>[2x]SNVPHKSSLPEGIRPSTVLRIRGLVPPNASRFHVNLLCGEEQGSDAALHFNPRLDTSEVVFNSKEQGSWGREERGPGVPFQRGQPFEVLIIASDDGFKAVVGDAQYHHFRHRLPLARVRLVEVGGDVQLDSVRIF

pmcHuman galectins (GAL) are oligomeric β-galactosidase-binding lectins assembled from small (∼15 kDa) protomeric carbohydrate recognition domains (CRD). Among prototype galectins, galectin-7 (GAL-7) is recognized for its preferential expression profiles in normal epithelial cells. For example, while extracellular GAL-7 can trigger apoptosis of activated T cells following binding to glycoreceptors via its GBS, it can also bind E-cadherin on epithelial cells independently of its GBS. In this work, we studied the impact of homodimer interface mutations on the induction of Jurkat T cell apoptosis, allowing us to positively and negatively modulate the biological activity of GAL-7 by designing a covalent disulfide bridge (G16C) and destabilizing mutation (G16S) to control homodimer strength, stability, and biological activity.

To examine whether these functional changes are rooted in structural perturbations at the molecular level, we solved the X-ray structures of lactose-bound WT GAL-7 and that of variants G16C and G16S in their apo and holo states. In contrast, our omit maps clearly show the presence of a bound lactose molecule in the GBS of both protomers within the WT, G16C, and G16S complexes. However, since Arg71 is located at the crystal contact surface, this dissimilarity could easily be an artifact of crystal packing. Lactose positioning within the GBS also remains analogous for WT GAL-7 and G16X variants, preserving the vast majority of the previously described polar interactions. Our results show that α-lactose-binding affinities (KD) were found to be similar for WT GAL-7 and G16X variants. Closer thermodynamic investigation illustrates that although WT and G16C exhibit very similar entropic (ΔS) and enthalpic (ΔH) contributions to ligand binding, variant G16S shows significantly altered ΔH and ΔS contributions relative to the two more stable WT and G16C forms of the protein, in line with the lower stability observed in variant G16S. In comparison with holo WT, holo G16X structures also exhibit higher Cα B′-factor values in loop 1, especially for residues Ile13, Arg14, and Pro15, which are located near the site of mutation. Besides loop 1, holo structures of G16S and G16C exhibit increased conformational variations in residues 37–46 (loop 3) relative to WT, a structural element neighboring the GBS. In the presence of lactose, loop 5 Cα B′-factor values decrease in WT, while conversely increasing in G16X variants. The shortest pathway between the two G16S opposite GBSs also exhibits a similar weight value of 0.27 and involves the same sequence of residues, but transposed to the other protomer: N62(B)-F61(B)-Y106(B)-A104(B)-D103(B)-R20(A)-V88(A)-F50(A)-H49(A). These results suggest that the primary interaction network connecting the GBS of each protomer is conserved in G16X mutants, although transposed between the A and B protomers in G16S.>[2x]GGGAAGAUAUAAUCCUAAUGAUAUGGUUUG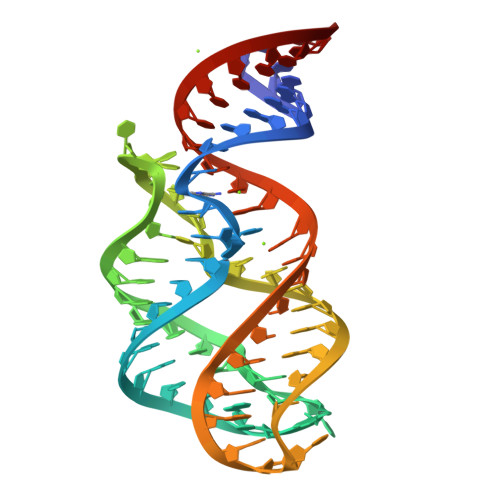GGAGUUUCUACCAAGAGCCUUAAACUCUUGAUUAUCUUCCC> HMAEIYLAGGCFWGLEEYFSRISGVLETSVGYANGQVETTNYQLLKETDHAETVQVIYDEKEVSLREILLYYFRVIDPLSINQQGNDRGRQYRTGIYYQDEADLPAIYTVVQEQERMLGRKIAVEVEQLRHYILAEDYHQDYLRKNPSGYCHIDVT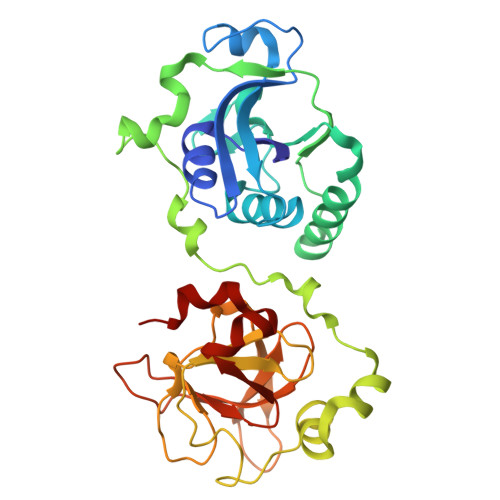DADKPLIDAANYEKPSQEVLKASLSEESYRVTQEAATEAPFTNAYDQTFEEGIYVDITTGEPLFFAKDKFASGCGWPSFSRPLSKELIHYYKDLSHGMERIEVRSRSGSAHLGHVFTDGPRELGGLRYCINSASLRFVAKDEMEKAGYGYLLPYLNK>MKILSKSIEKMQSDTQEANDIVTLANLQYNGSTPADAFETKVTNIIDRLNNNGIHINNKVACQLIMRGLSGEYKFLRYTRHRHLNMTVAELFLDIHAIYEEQQGS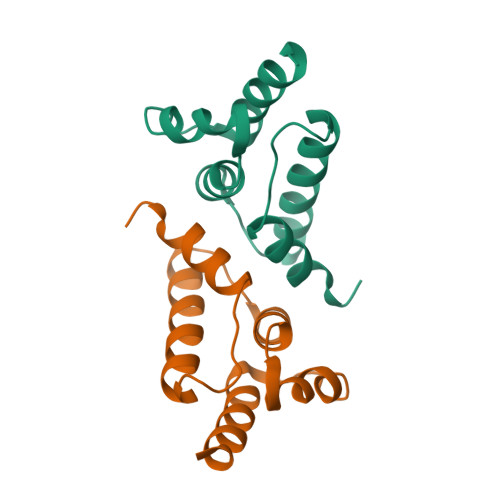RNPLEHHHHHH[3x]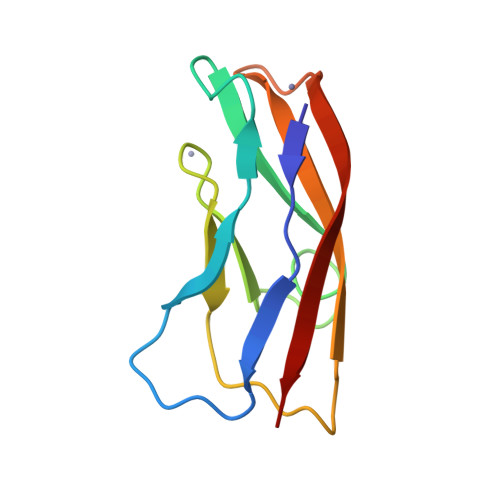> SILATPILIPENQRPPFPRSVGKVIRSEGTEGAKFRLSGKGVDQDPKGIFRINEISGDVSVTRPLDREAIANYELEVEVTDLSGKIIDGPVRLDISVID>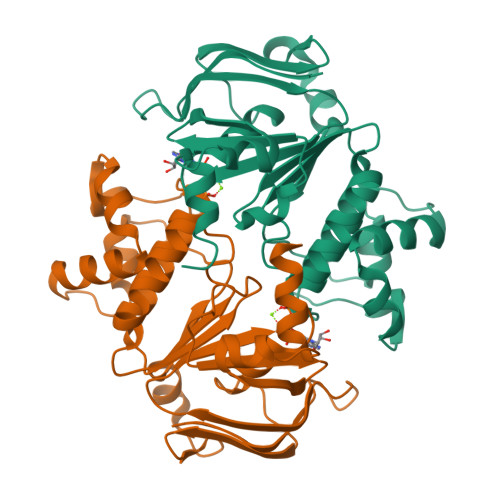[4x]DITFRNIRFRYKPDSPVILDNINLSIKQGEVIGIVGRSGSGKSTLTKLIQRFYIPENGQVLIDGHDLALADPNWLRRQVGVVLQDNVLLNRSIIDNISLANPGMSVEKVIYAAKLAGAHDFISELREGYNTIVGEQGAGLSGGQRQRIAIARALVNNPKILIFDEATSALDYESEHVIMRNMHKICKGRTVIIIAARLSTVKNADRIIVMEKGKIVEQGKHKELLSEPESLYSYLYQLQSD In our previous work, using a combination of computational and in vitro screenings we created a panel of FAPs from bacterial lipocalin Blc (named DiBs) capable of recovering the fluorescence of synthetic analogs of green and red fluorescent proteins’ chromophores. The lipocalin fold contains a single eight-stranded continuously hydrogen-bonded antiparallel β-barrel complemented by an α-helix. Fluorogen-activating proteins (FAPs) are a group of unrelated proteins capable of binding to non-protein ligands (fluorogens) and increase the fluorescence quantum yield and/or change spectral properties of these ligands. Here we report on DiB-splits, a self-assembling FAP split system which has been inspired by the domain-swapped structure of a full-length DiB protein.

Our attempts to structurally characterize other DiB proteins in apo and bound states resulted in obtaining protein crystals of DiB3 in the apo form at low pH conditions (pH 3.5) which diffracted to 1.6 Å. The asymmetric unit contains only one protein chain. However, it forms a biological assembly (dimer) with a crystallographic symmetry mate. The intertwined dimer is caused by domain swapping: each of the two Blc-like eight-stranded beta-barrel folds is created by the N-terminus of one of two polypeptide chains and the C-terminus of the other. While DiB3 was previously successfully used for in cellulo protein labelling, we proposed that the observed domain swapping was driven mainly by the very low pH conditions of the crystallization buffer rather than the private DiB3 mutations (V74F and L141Q). To further evaluate this assumption, we calculated the interaction energies between N- and C-termini fragments of the wtBlc, DiB1, and DiB3 proteins using Rosetta38. Despite the fact that wtBlc protein seems to be slightly more stable, DiB3 is not an outlier, suggesting that the introduced mutations are unlikely to cause the domain swapping. Independent from the reason that caused domain swapping in the crystal, we reasoned that the DiB3 protein as well as other mutants might have two relatively autonomous and stable parts (residues 1 to 108 and 114 to 177). In our case, however, the obtained DiB3 structure is pointing to a potential cleavage site. In this study, inspired by the obtained domain-swapped crystal structure of the DiB3 protein in its apo state, we designed and characterized a novel DiB-split FAP system.

> MGGSHHHHHHLESTSLYKKSSSTPPRGVTVVNNFDAKRYLGTWYEIARFDHRFERGLEKVTATYSLRDDGGLNFINKGYNPDRGMWQQSEGKAYFTGAPTRAALKVSFFGPFYGGYNVIALDREYRHALVCGPDRDYLWIQSRTPTISDEVKQEMLAVATREGFDVSKFIWVQQPGS> MSYSQTINSLVEVVLVLVPSLVGIAYVTVGERKTMGSMQRRLGPNAVGIYGLLQAFADALKLLLKEYVGPTQANLVLFFLGPVITLIFSLLGYAVIPYGPGLAVNDLSTGILYMLAVSSLATYGILLAGWSANSKYAFLGSLRSTAQLISYELVLSSSILLVIMLSGSLSLTVIVESQRAIWYILPLLPVFIIFFIGSVAETNRAPFDLAEAESELVSGFMTEHAAVIFVFFFLAEYGSIVLMCILTSILFLGGYLLISLLDIIYNNLLSWIVIGKYIIFIFPFWGPVFIDLGLYEIISYLYNAPTVEGSFYGLSLGVKTSILIFVFIWTRASFPRIRFDQLMSFCWTVLLPILFALIVLVPCILYSFNIFPVNISLL;> MIMISILSLLLSTSVTLRRDMSILFNRISIIALAYCILHDTMSLSFISKGIGLHGGLLHITNLTQIFHIFIFIISILILQLTSFYPRKVWIPEYSSLKDIFFNKILYYRTKIINKMGEHMKIIEYPLILLFVISGAVFLISTNDLVSIFLSIELQSYGLYLLSTIYRNSELSTTGGLIYFLLGGLSSCFILLGTSLLYVNSGTTSLDGLYILNSISDVNPVVAGVGEDGGLTSWYKPYYLNFSLLIFSIGFLFKVSAAPFHFWSPDVYDAIPTIVTTFVAIIAKISIFIFLLELVYYTNSNANSYLSEFSWTYALLISSLLSLIIGTVVGLTQFRIKRLLAYSTISHVGFILLALSVSSIESTQAFIFYLIQYSISNLNAFFILITIGFSLYGYVTNNKEYKSLLDKNNSPIQLISQLKGYFYINPLLSLSLAITIFSFVGVPPLVGFFAKQMVLSAALDNGYIFLSLIAIITSVIGAVYYLNVIKEIFFYSPEHEVNPVLNESDSNFSLRILNEKNVLIRSVLLKGRNIFISSPFSITISIITNVILLFIFMNKEWLSMGTILVQILFSA;> MSAMSIYIIFVSIIAILFLAIDLIFAPHNPYKEKLSAFECGFHSFSQSRSPFNISFFIYGLVFLLLDLEILLLYPFAVSEYVNSAYGLAAALIFIGIITIGFVYELGHDALKVHSRQNISTKDLKSSVVISYLGNINNDSVNLHIK;> MSLLYVLLIIPIIGIFLISTIDSFYPVTNTNIVLNKKFFRGFNDARQPIKYLYFSEGESFNIENKEDSFFNVSYYKKIALITTILNLIVSLIIYILFDFSNNQFQFIQENLDLSFYDIYLGVDGVSIYFVLLTTIIMPIALVSNWNSITNNIKSYLIIMLLLETLLLAVFLVLDVLLFYIFFESILPPLFILIGLFGSSNKVRASFYIFLYTLLGSLFLLLSILTMSSIVGTTYFDVLLKSSFEYTTQLFLFFGIFIAFAVKTPVWGLNSWLLRAHVESPLGGSIVLAAIVLKLSLYGVFRLILPILPQASLNLTYIVYAIGAITVLYASFSTLR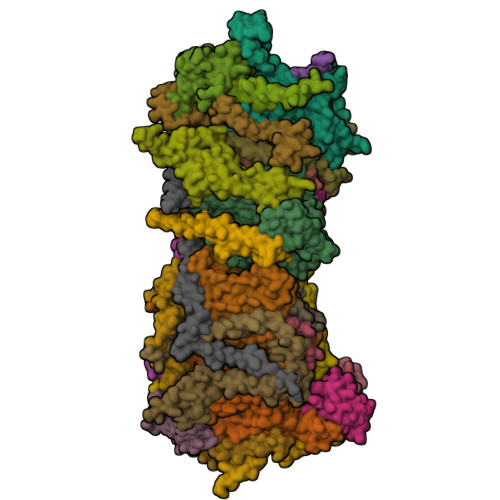TVDVKELIAYSSVAHAAIYLMGVFSNTIQGLEGAILLGLAHGFVSSGLFICAGGILYDRTGTRLIYFFRGLTQIMPLFSLFFFILCLGNAGTPLTLNFVGEFMSLYGTLERLPIAGMLASTSIIFSAAYSIYMYNRIAFGGSVSLYFIDCFRDLTKREFFILFTLVSFTVILGIYPSFVLDGLHYNISSVVYGIEPNASYLTQGGNL;> MYLSIIILPLLGSVVSGFFGRKVGVSGAQLITCSSVIITTILSIIAFFEVGFNNIPVTINIFRWIDSEWFIINWGFQYDSLTVSMLIPVLIISSLVHIYSISYMSSDPHNQRFFSYLSLFTFMMIILVTANNYLLMFVGWEGVGVCSYLLVSFWFTRIAANQSSISAFLTNRVGDCFLTVGMFAILWSLGNLDYATVFSLAPYINSNVVIIIGICLLIGAMAKSSQVGLHVWLPMAMEGPTPVSALIHAATMVTAGVYLLMRSSPLIEYSSTVLLLCLWLGAITTVFSSLIGLFQQDIKKVIAYSTMSQLGMMVLSIGLSSYNIALFHLVNHAFYKALLFLGAGSVIHAVADNQDFRKFGGLISYLPLTYSVMLIASLSLVAFPFMTGFYSKDFILESAYGQFSFSGVAVYIIATIGAIFTTLYSVKVLYLTFLSNPNGPRTYYRLAIDNFFSAQAIKSYKPAHEGDFFLTLPLVILALFSIFFGFITKDIFIGLGSNFFVDNSLFIHPIHEIMIDTEFAVPVLFKLLPFIFTISFSVIALTLSELLSELVIYFKFSRFGYNIFGFFNQRFLIEFFYNKYITNLILNLGGQITKILDKGSIELFGPYGLERGLVKLSKNISSLSTSHVTTYALYILVGFILYLIYNNLLLDYSYLLLIIILLLLLMMIGESNSEDVTLH;> MNSQISLLLLKEIYTNGSTHIMLDILSVLAVISGICVIISKNPIVSVLHLIGLFAYVSFYLILIGLNFVGLSYLIVYIGAVSILFLFILMLINIRTSELQSNTSNSIPLTILVGIIISSFLFKMLPYGVIISNQFNSSNLNENLYTIQIVGGEDNNINNINTDKNDLFFITSKIWDGALAENNHISSIGNIMYTNYNVWLILASFILLLAMVGAIVITIKPRKI;> MATDAAETSRRATREEMRDAKVPLAYRDSCAHLLIPLNRCRYETYYLPWKCEDERHSYEKCQYLEFKKRVQKMEELREAKGGARSN;> MASGYGLNGGPSRCFPFWQELLACYVTNSSEDNPDGKNKCIPVMEDYYECLHHRKEAARVRALQAAYREAEAKKLQENPPTAGQIRNLGLLNKEEDTKKVHCATATQQWMKMCFALSAKMPCLRGIEVFLTTRPDNEKIPEYPHPEGTSARVICGQHLIRSPSLASNLSNSAITPPSSFSPRKANPLVSVYLPSVPGTPFTINYKISQVPPEPCKYLFFRLYINARPMVSWGIDPHSRPYGKVIKSLWLPSDDRYRGLVGFEKRSFVFLPGEEFKSVAEDGGLIEVQVFRAKDRRARTPKLETFRFRDNYGIAAPSIGLLDKPQNAFFYDWLLIDPKDEPFAKFRMHYRSWRNLKSLNLIPSSEWELLLAVSPKALRTAASTGKIEKPTSPAFSDSDSDDSLCSATDSDECVFDDHSKKTKSNRSKESPFAFLNSPPERFRAMAPSSEKLPQPSKLLRDSQRAPYQSRPLPELPVEAGVNSTGLNPPSVKVAADLRRKPSATSMESNAVSITPSLLRCMEEGTLDLEKAEVGIAKLVKVAASGSEPSSSSSSATQLTVSAVREVELRPPQPERKGGLPMDYSFSDYEKSSQSSFGDDERMSNISDMEEKPFPAPPTCYLPTTGSGLERELAMFDSPSPSPVPYSAMEPPVTPSPSSTPYKTKLGRKPLLFSRRLGLFSPRKSLPSDFLLGQAKKLVVEEETTNSNVSLAFGELTVTDMRAESPSPAPKGKPLRRFSTIRVEEISIKEKRPLFNSLRRIASASPRKLAGRVLSMDLGKKGGEEKEG;> MPVPFETLIPYGIIIAMFGVTGAGMAKVRHMFNGDKRHRWSVDQWDKQQMERDRRLTGHLRGQTDNPIAPPGFEFNNPWKVXXXXX;> MAPIEEEHEHYHPKDAVHLGLKGAAVVGGIGLLFAAVRTSLARKNVGPWAIFTRNGKLAATFAAVGGAYDFTRAAAANLREKEDWVNNGIGGLFAGATMGLTTGRIPRVLGFAALTGVVLATAEYAGSGLRGVFKRDVDEYERKEFLRKNRRRPIEETLAEIGEGRGIKPPGYYERRAQRLKEKYGVDINPVCADPDQA;> MNITLILFLIGILGFVLNRKNIILMLISIEIMLLSITFLILLSSLNMDDIIGQTYAIYIIVVAGAESAIGLGILVAFYRLRGSIAIEYK;> MFRSAVLRSAAAATRTTIRSIPPAAAKKFAVAPVSRVTSFIPKTASWQVIRCYASNEGLQKVEVYERIKSLLAGFDKVNDPNNITETAHFANDLGLDSLDTVEVVMAIEEEFSIEIPDKDADQIHSVDKAIEYILRQPDAH;> MSNRQAALSLYRRALKLALDWTVHRNLWRGQALYIRSLFEKNRNVTDPRLQRALLKETEKLLEKWKHPDPYCPPTAPGGSKYERNLPVPNLEPPPPLKF;> MDGGPPTFAFRPTARQAPGKLSSAPVTTRLAAAALSRASTVSSKALTPARFRFFSTTQRRAGGHGMQYDPPTGWLWGVRPGEKYQNEGWEGPFFYGFWGSLIVFAIAYAYKPDTSIQTWALEEARRRLEAEGILEDPNPTKKE;> MATRKPAFNQHVLLDTTPLPDSIPKVKEIGASSAPLLSASFFIGARCKDYNDDYMQCKNENPGRGEFECLKEGRRVTRCARSVLKDINTHCLEQFRAHWQCLDNNNQQLWQCRPAEWKLNKCVYENLKLEKVIPDQPKNSTPVHLRQRQIFAHHAIPPWERPFIPGQPEPQLPAGIEIPEKYKNQS;> MPQDMPPPGGYEAVQYKRNLPSRGLFRPRPLLAGAAVLMLYGWYKLVKGIREQNELAREKMWARIHLIPLLQAEEDRDHVRRYLADQAREKGLLGENIKVYNSDRYVRPTFAVTPSKPAQE;> MSNTPTQTYQFPSKTVKTDYPLIDNDPHFTRVIRYARPSDYAHGLAAAAAGPAALWLMERISPSQVGRGGFAKAMRLAGFIGLAGGFLYFYQRSILRFYGMSENAREVEMDMREMTDRVKAGLPLYGESRLSPAMQGVAARQSRYSALFFGVMPWFNFVNHNQHGVDTAKYYQQAERELEAERLAREQAQQ;> MLSRRLVRAVAPLRSPVLPAARRLPLIQQRTFLPEAMVGRSKIDEKYPDSDYPTLTDKEDPDMNGGYINPPRIKRQFRDPHADWWDKQERRNFGEPVHEDHDILGMFSPYEYTWITPGKGLFQIGLFIASFLGLCYVVKLTYPDRVSYPREFEGGLERELGGAGAVRAFLCLDDEIMWMVSLYCLPASKLISSPVALQDKSTSSASAMRYDDWDVILFPTGRDSKIPFKEFKVACHVVPDIELAHLHGAVGSPVMTCFVPSLPPGTPFQVSIHCWRRPEISQFARTYSKNPDLVKFEARVTLDGRLVASAILDRDVNGPHLITSTFEFTKTGELERLTFPAFRQEILRQNHWHPGDDLGRIKVIISEGFPRDSLTVPIERVKNIVTFSFQHAPLGKIPGIAWPNPGMWRRPTPNPAVSVPTYFPGDGAESHAHSPGKRSLLLKGIRNHGFPSTVIPGSIFHHQSNPAGLLNPPGFKVPHFSASNPSVPNIFSPHDPFAEPTYRDWMSSITNVQAGDFWDGRTTWPINPRNFHKSDTIMADCPSQGGDPMQISGSSLEDDPLRLKAPQNTPTEGGEGPNPGAQFAHPIPSELTADLESALSQSLLNQAPTSAISQRNFPMPHSDGLSRKEGRQVSLGQGTSAQMPSTSSSMEARRLSQALFGMNNLPIEASVNNGVSASVTPLFAANQRSVNNPLVATFGSAILSQGSTNPSGTEQSTDTTATTTAAAAAAVTDVQVEPPAPTSNAANESVINLTSGTSSTSTVHANVPTSVSKRPRNFTPASARVIDEEDEPRRTSPQVQVGGFAETTSVEESIQ;> MVNRILFWTGFGLAVRFWQLGIEMRPFFNRKSLWAYPLFGGVGASFGYWLQSIDEKQTKMLEERKQAILEKRARRAQRQAEAAATAPSPSAQEA;> MQPTRILRNNGEKPNITGFDMREFLRHTKTPTYDPWERHEAWRYTGRFSRFNRFKGALPGFGIATVAFTAYCVFEHFFLKDDHHGHHGEKEHH;> MPTPESEAFLAKKPQVPPTFDGVDYEDNKRLKQAQDAIIREQWVQVMMGRLVREELSKCYYREGVNHLEKCGKLRERYLQLLANAKVKGYLFEQQNYWSKENQQQ;> MAGGGQHVSRVHRFLATGLGASMWFWIFYRAKKDGPVLLGWKHPWD;> MSATTPRFWSTPLKYCRWAARERPALFFSVVIGALGPVTLATVPPLRRLIGDVDAAPIPLTYPIPPGPRKQLKGYDDDTEDN;> MGGGPKIPYPKHVWSPAGGWYAQPANWKQNTAIFGLVIFGITAMVWKYSAEHEVRHKMPEPDRFYPSRYWVKQIKDYERAQKEKQQNNTEASS;> MAGLQHYKIAMDPALVRLGSMISNRYKYFRWTKRTALVSFMYVVVVPSTIGYLAYKTDGLWDLRAKRRGDLISER;> MLALRQRAALLARRVRPTVVVPRNARTYASSHDHDHHDHHHDHGHNVEEPLGAAFYIAVGGIASSFVIYNISRPGPNGEPSSLHKWFSKISDYKDEWETRNTLMAAALEQAAHDKHLLLTAERSRHIELKYPEVFSHGSPFNVPAGFYPNLDHVIEHYRKQHLEEEERKAKKLAAAAAAASEAR SMYD2 is a lysine methyltransferase that catalyzes the monomethylation of several protein substrates including p53. The SMYD enzymes display a distinct protein architecture in which the SET sequence is split by a zinc finger containing the myeloid translocation protein-8, Nervy, and DEAF-1 (MYND) motif followed by a cysteine-rich post-SET domain. Like SMYD3, SMYD2 also targets a number of histone and non-histone substrates including histones H3, H4, and H2B; p53 (15); retinoblastoma (Rb; Refs. 16 and 17); HSP90 (18, 19); estrogen receptor α; and poly(ADP-ribose) polymerase and is implicated in both cancer and muscle development. SMYD2 is overexpressed in a significant percentage of esophageal squamous primary carcinomas, and that overexpression correlates with poor patient survival.

A 1.63-Å resolution crystal structure of SMYD2 in complex with LLY-507 shows the inhibitor binding in the substrate peptide binding pocket. LLY-507 binds in the substrate peptide binding site of SMYD2 with the pyrrolidine group ensconced in the lysine pocket formed by the side chains of Phe184, Tyr240, and Tyr258. The nitrogen atom of the pyrrolidine makes a hydrogen bond to an ordered water molecule, whereas the oxygen and nitrogen atoms of the methylene amide linker form hydrogen bonds to the main chain amide nitrogen of Thr185 and a bound water molecule, respectively. The benzonitrile group makes a C–H···O hydrogen bond to the main chain carbonyl of Gly183 with the nitrile group oriented toward the solvent. The piperazine packs against Asn180, and makes C–H···O hydrogen bonds to the Asn180 side chain. The indole stacks between the side chains of Lys145 and Asn180. The phenyl linking the benzonitrile to the piperazine sits in a pocket formed by the side chains of Thr105, Thr145, Asn180, and Ser196 as well as the backbone amide units of Val179, Gly183, and Phe184. The high resolution structure of SMYD2 in complex with LLY-507 reveals the significant overlap of the ligand binding site with the substrate peptide binding site and provides a plausible rationale for the selectivity of LLY-507 for SMYD2. LLY-507 potently inhibited the ability of SMYD2 to methylate p53 peptide with an IC50 <15 nm.

> MRAEGLGGLERFCSPGKGRGLRALQPFQVGDLLFSCPAYAYVLTVNERGNHCEYCFTRKEGLSKCGRCKQAFYCNVECQKEDWPMHKLECSPMVVFGENWNPSETVRLTARILAKQKIHPERTPSEKLLAVKEFESHLDKLDNEKKDLIQSDIAALHHFYSKHLGFPDNDSLVVLFAQVNCNGFTIEDEELSHLGSAIFPDVALMNHSCCPNVIVTYKGTLAEVRAVQEIKPGEEVFTSYIDLLYPTEDRNDRLRDSYFFTCECQECTTKDKDKAKVEIRKLSDPPKAEAIRDMVRYARNVIEEFRRAKHYKSPSELLEICELSQEKMSSVFEDSNVYMLHMMYQAMGVCLYMQDWEGALQYGQKIIKPYSKHYPLYSLNVASMWLKLGRLYMGLEHKAAGEKALKKAIAIMEVAHGKDHPYISEIKQEIESHEGHHHHHH Furin is the most prominent member of the human proprotein convertases (PCs), a family of 9 serine proteases possessing a Ca2+ dependent subtilisin-like protease domain. The PCs catalyze the posttranslational maturation of many proproteins thereby contributing to a variety of physiological processes. Furin and six additional PCs (PC1, PC2, PC4, PACE4, PC5, and PC7) cleave their substrates after multibasic sequences and, therefore, are often named as basic PCs. The proprotein convertase (PC) furin emerged as promising drug target for the treatment of numerous infectious diseases, cancer and cystic fibrosis.

In all complexes, the central dichlorobiphenyl-segment occupied a hydrophobic pocket in a similar manner, as described for furin in complex with various dichlorophenylpyridine-derived inhibitors. , This cryptic binding pocket was opened after a flip of the side chain of the furin residue Trp254 by approximately 180° and lined by the hydrophobic side chains of furin residues Leu152, Met226, Leu227, Val231, Leu240, Ala252 and Trp291. Additional contacts found in all complexes were a characteristic salt bridge between the piperidyl nitrogen on the left inhibitor arm (ring C) and the carboxylate of Glu236, as well as a polar interaction from the same nitrogen to the hydroxy group of Tyr308. Binding modes could be also determined for the asymmetric inhibitors 13, 26, 27, and 41. The electron densities of the central biphenyl core and the structurally similar left arms of inhibitors 13 and 26 were well-defined. The trifluoroacetamide and acetamide groups were involved in two identical water mediated polar contacts between their amide NH and the carboxyl group of Asp264 and its carbonyl oxygen to the backbone NH of Asp233. In contrast, in both structures a sufficient electron density could be only obtained for the first ring D of the right inhibitor arm. This suggests a high flexibility of the terminal ring E in these inhibitors. The bound conformation of both inhibitors was nearly identical.

> DVYQEPTDPKFPQQWYLSGVTQRDLNVKAAWAQGYTGHGIVVSILDDGIEKNHPDLAGNYDPGASFDVNDQDPDPQPRYTQMNDNRHGTRCAGEVAAVANNGVCGVGVAYNARIGGVRMLDGEVTDAVEARSLGLNPNHIHIYSASWGPEDDGKTVDGPARLAEEAFFRGVSQGRGGLGSIFVWASGNGGREHDSCNCDGYTNSIYTLSISSATQFGNVPWYSEACSSTLATTYSSGNQNEKQIVTTDLRQKCTESHTGTSASAPLAAGIIALTLEANKNLTWRDMQHLVVQTSKPAHLNANDWATNGVGRKVSHSYGYGLLDAGAMVALAQNWTTVAPQRKCIIDILTEPKDIGKRLEVRKTVTACLGEPNHITRLEHAQARLTLSYNRRGDLAIHLVSPMGTRSTLLAARPHDYSADGFNDWAFMTTHSWDEDPSGEWVLEIENTSEANNYGTLTKFTLVLYGTASGSLVPRGSHHHHHH> LSECKTGNGKNYRGTMSKTKNGITCQKWSSTSPHRPRFSPATHPSEGLEENYCRNPDNDPQGPWCYTTDPEKRYDYCDILECEEECMHCSGENYDGKISKTMSGLECQAWDS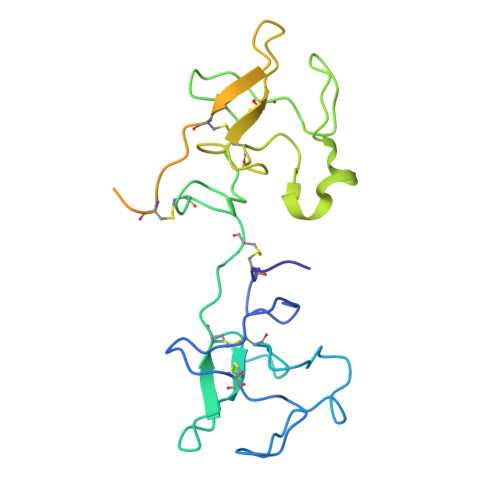QSPHAHGYIPSKFPNKNLKKNYCRNPDRELRPWCFTTDPNKRWELCDIPRCTTPPPSSGPTYQCLKGTGENYRGNVAVTVSGHTCQHWSAQTPHTHERTPENFPCKNLDENYCRNPDGKRAP> DAASHAGTTYIFSKGGGQITYKWPPNDRPSTRADRLAIGFSTVQKEAVLVRVDSSSGLGDYLELHIHQGKIGVKF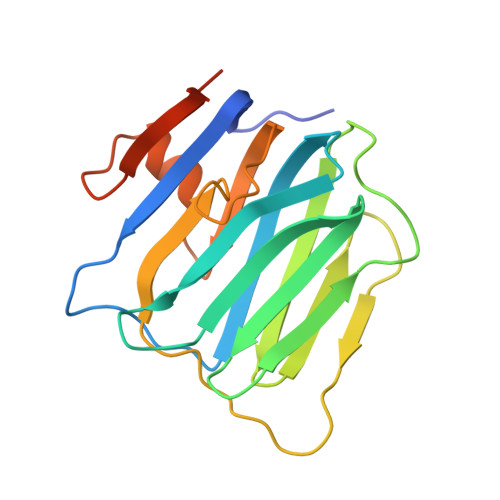NVGTDDIAIEESNAIINDGKYHVVRFTRSGGNATLQVDSWPVIERYPAGRQLTIFNSQATIIIGGKEQGQPFQGQLSGLYYNGLKVLNMAAENDANIAIVGNVRLVGEVPGSHHHHHH>SNAMKEALATGSEAWWRTKTGPEWIREKDGNYRVTFWWRDPQGNETHSPIRRVWVYITGVTDHHQNAQPQTMARIAGTDVWRWSTALSANWRGSYCFIPTERDDVFAAFAPGETPDRNVLREGWRQLLPQAIADPLNSQSWRGGRGHAVSALEMPDAPLQPGWDRPETPYSPPLMMQWHSERLGNSRRVWILTTGDEAPEERPLAILLDGQFWAENMPVWPALASLTHQRLLPGAVYLLIDAIDTQHRSQELPCNADFWLA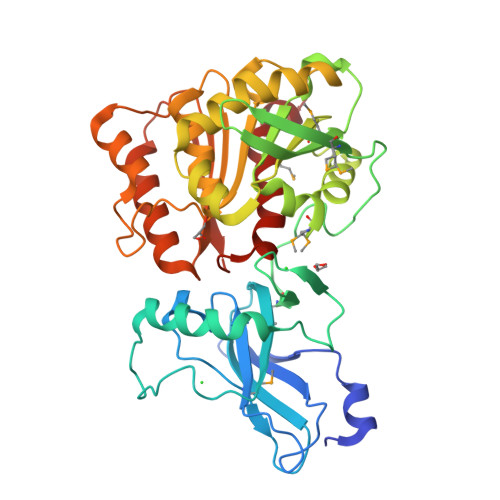VQQELLPQVRAVTPFSDDAGRTVVAGQSFGGLSALYAGLNWPTRFGCVLSQSGSFWWPHRITPPEGEVITRLKTGALCARGLRIVLEAGVREPIVFQANQALYAQLNTSQQSIFWRQVDGGHDALCWRGGLTQGLMLLWQPLIDTL[2x]> AMKKIEMIEISQNRQNLTAFLHISEIKAINAKLADGVDVDKKSFDEICSIVLEQYQAKQISNKQASEIFETLAKANKSFKIEKFRCSHGYNEIYKYSPDHEAYLFYCKGGQ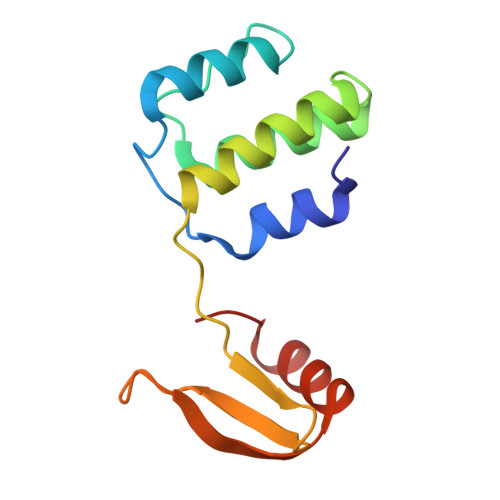GQLNKLIAENGRFM>[4x]STTLTRQDLNFGQVVADVLCEFLEVAVHLILYVREVYPVGIFQKRKKYNVPVQMSCHPELNQYIQDTLHCVKPLLEKNDVEKVVVVILDKEHRPVEKFVFEITQPPLLSISSDSLLSHVEQLLRA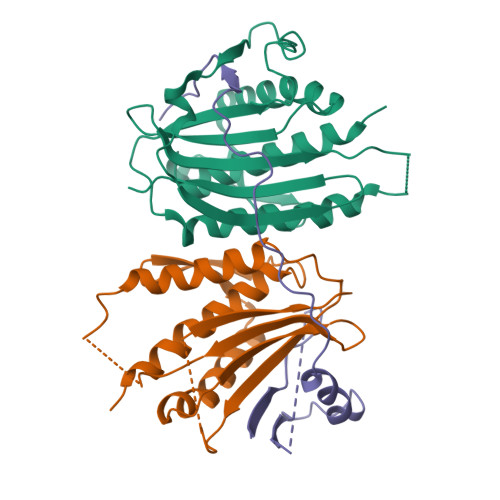FILKISVCDAVLDHNPPGCTFTVLVHTREAATRNMEKIQVIKDFPWILADEQDVHMHDPRLIPLKTMTSDILKMQLYVEERAHKGS;>[2x]MSQVHIFWGAPIAPLKGSGSGSGSGSGSGSGSTTEVILHYRPCESDPTQLPKIAEKAIQDFPTRPLSRFIPWFPYDGSKLPLRPKRSPPASREEIMATL4-(methylamino)benzoic acid | C8 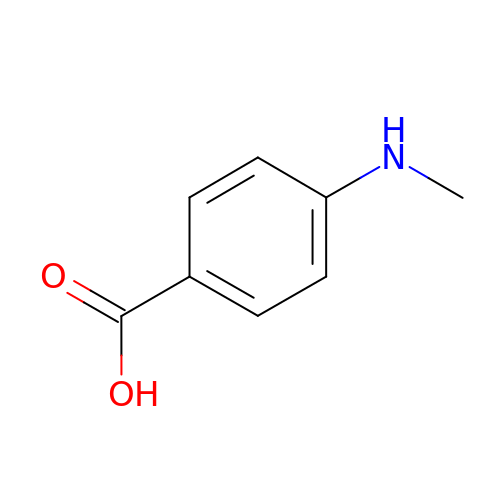H9 N O2 | ZVIDMSBTYRSMAR-UHFFFAOYSA-N> MHHHHHHSGGSRSEAHSNSIGILAMHNNIIRDFTKIASNNIDLAIEDITTVDHSLNSIYSLLKSHHMWGHINSTVKQHLMIIVKLINNNALGLASSEIIFLFNETNLFQAHSLKNILLADFSTWNDYYLSNLKILALQIILKRKLVDEYLPHILELFSHDKRYLLKDPNLKAHALTKIVLSFFSVTTSCKVLFGLKFLQYIKQFKLPFKKFISNITVECFSKNLLHKNYLEMGPNKIYLNSFYLSYSMLYDGLDKIMLLDILSYEETTEVQRAIKSKKEFNEYCNMSENRLLWSCISVDDLNVILENATNFLQNKGKHISATLKCLVCLWSTIRLEGLPKNKDILRQFDCTVIYINSNIKSINDESAAALLSELLGVLSEICIDYKEPKRLSNIISVLFNASVLFKSHSFLLKTANLEISNVLISNDSKTSHRTILKFEKFISSAQSAQKKIEIFSCLFNVYCMLRNDTLSFVFDFCQNAFIHCFTRLKITKFIEFSNSSEIMLSVLYGNSSIENIPSENWSQLSRMIFCSLRGIFDLDPLELNNTFDKLHLLNKYELLIRIVYLLNLDMSKHLTTNLSKITKLYINKWLQKSDEKAERISSFEMDFVKMLLCYLNFNNFDKLSIELSLCIKSKEKYYSSIVPYADNYLLEAYLS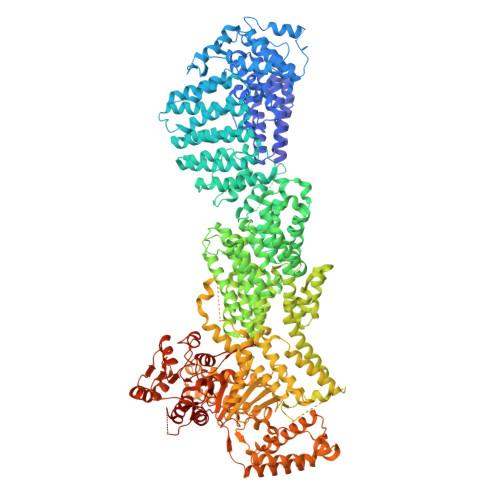LYMIDDALMMKNQLQKTMNLSTAKIEQALLHASSLINVHLWDSDLTAFQIYFGKTLPAMKPELFDINNDHNLPMSLYIKVILLNIKIFNESAKLNIKAGNVISAVIDCRKAQNLALSLLKKKNKLSQGSRLALLKSLSFSFFQLIKIHIRIGSARDCEFYSKELSRIISDLEEPIIVYRCLHFLHRYYMITEQTCLQNITLGKANKAFDYLDAEADITSLTMFLYDNKEFVKLEQSLVLYFGDQLEKTFLPNLWKLHLGKDIDDSICLSEYMPKNVINRVHNMWQKVMSQLEEDPFFKGMFESTLGIPSSLPVIPSTMPNNILKTPSKHSTGLKLCDSPRSSSMTPRGKNIRQKFDRIAAISKLKQMKELLESLKLDTLDNHELSKISSLSSLTLTILSNITSIHNAESSLITNFSLTDLPRHMPLLFDKVLNNIDNKNYREFRVSSLIAPNNISTITESIRVSAAQKDLMESNLNINVITIDFCPITGNLLLSKLEPRRKRRTHLRLPLIRSNSRDLDEVHLSFPEATKKLLSIINESNQTTSVEVTNKIKTREERKSWWTTRYDLDKRMQQLLNNIENSWFNGVQGFFSPEVVDNSLFEKFKDKFYEILHQNLPSRKLYGNPAMFIKVEDWVIELFLKLNPQEIDFLSKMEDLIYFVLDILLFHGEENAYDEIDFSMLHVQLEEQIKKYRATMTTNSIFHTFLVVSSSCHLFPWECLSFLKDLSITRVPSYVCLNKLLSRFHYQLPLQVTIEDNISMILNPNGDLSRTESKFKGMFQKIIDAKPSSQLVMNEKPEEETLLKMLQNSNLFVYIGHGGGEQYVRSKEIKKCTKIAPSFLLGCSSAAMKYYGKLEPTGTIYTYLLGGCPMVLGNLWDVTDKDIDKFSEELFEKMGFRCNTDDLNGNSLSVSYAVSKSRGVCHLRYLNGAAPVIYGLPIKFVS>MGSDKIHHHHHHENLYFQGTNLIVNYLPQNMTQDELRSLFSSIGEVESAKLIRDKVAGH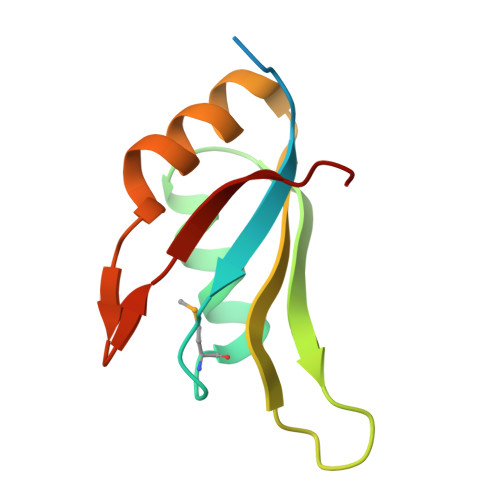SLGYGFVNYVTAKDAERAINTLNGLRLQSKTIKVSYARPS[4x]4-Borono-L-phenylalanine | C9 H12 B N O4 | 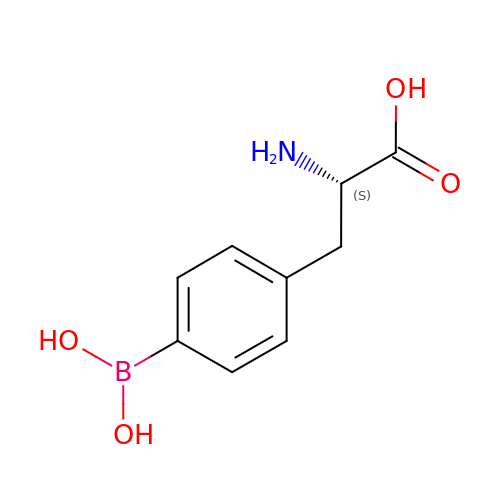NFIVJOSXJDORSP-QMMMGPOBSA-N> MFTKSGDDGNTNVIN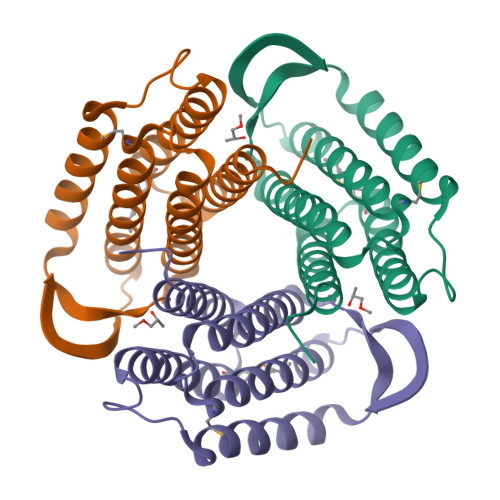KRVGKDSPLVNFLGDLDELNSFIGFAISKIPWEDMKKDLERVQVELFEIGEDLSTQSSKKKIDEKYVKWLEERTVEYRKESGPVKLFVIPGGSEEASVLHVTRSVARRVERNAVKYTKELPEINRMIIVYLNRLSSLLFAMALVANKRRNVSEKIYDIGKFW>[3x]MASLTVKAYL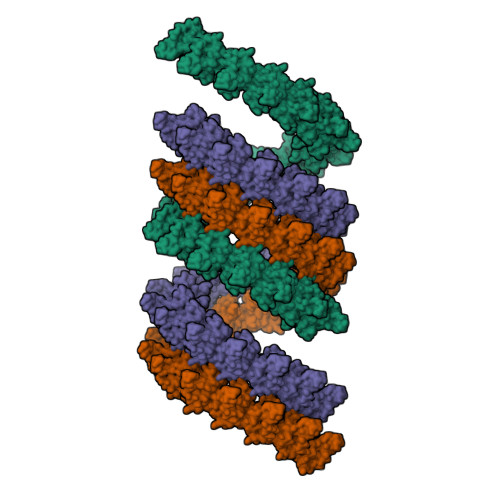LGKEDAAREIRRFSFCCSPEPEAEAEAAAGPGPCERLLSRVAALFPALRPGGFQAHYRDEDGDLVAFSSDEELTMAMSYVKDDIFRIYIKEKKECRRDHRPPCAQEAPRNMV(5Z)-5-(3,5-difluoro-4-hydroxybenzylidene)-2,3-dimethyl-3,5-dihydro-4H-imidazol-4-one | C12 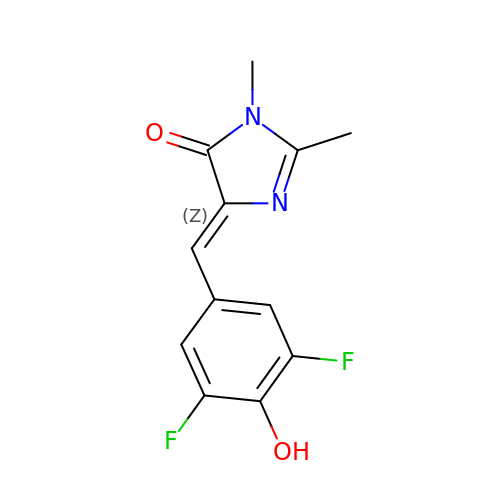H10 F2 N2 O2 | ZDDIJYXDUBFLID-YHYXMXQVSA-N>MNKDLKGLYAALLVPFDENGQVNEQ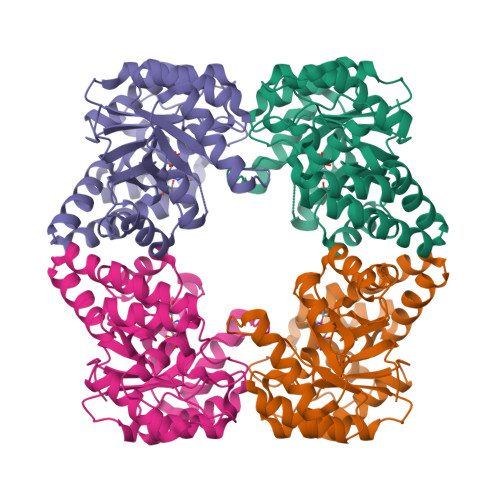GLKQIAQNAIETEELDGLYVNGSSGENFLLNTEQKKQVFKVAKEAVGDKVKLIAQVGSLDLNEAIELGKYATELGYDALSAVTPFYYPFTFEEIRDYYFDIIEATQNNMIIYAIPDLTGVNISIEQFSELFNHEKIVGVKYTAPNFFLLERIRKAFPDKLILSGFDEMLVQATISGVDGAIGSTYNVNGRRARKIFDLARQGQIQEAYQLQHDSNDIIETVLSMGIYPTLKEILRHRGIDAGLPKRPFKPFNEAHRQTLDQLIAKYDL[4x]>MMSETAPLPSASSALEDKAASAPVVGIIMGSQSDWETMRHADALLTELEIPHE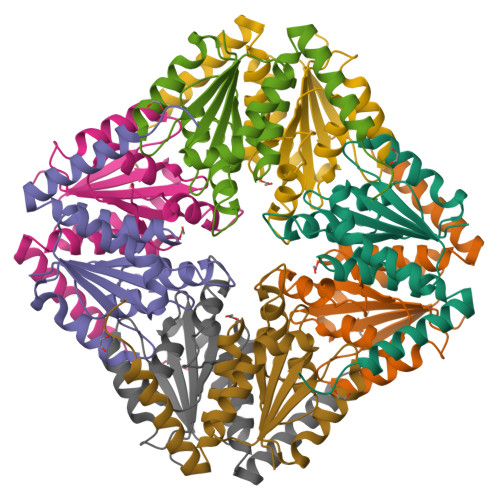TLIVDAHRTPDRLADYARTAAERGLNVIIAGAGGAAHLPGMCAAWTRLPVLGVPVESRALKGMDSLLSIVQMPGGVPVGTLAIGASGAKNAALLAASILALYNPALAARLETWRALQTASVPNSPITEDK[2x]3-METHYL-1,2-DIHYDROQUINOLIN-2-ONE | C10 H9 N O | 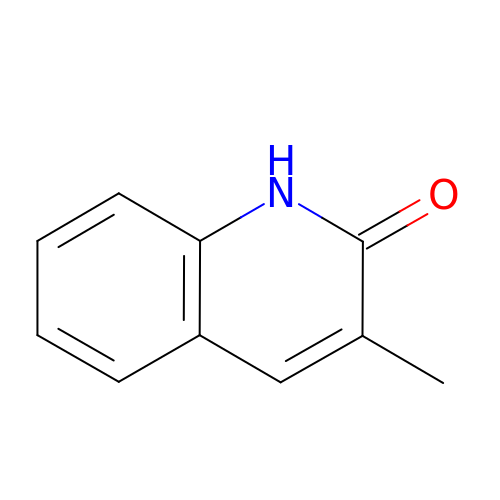POYSUXIHCXBJPN-UHFFFAOYSA-N>[8x]HHHHHHLEVLFQGPMKYTKLE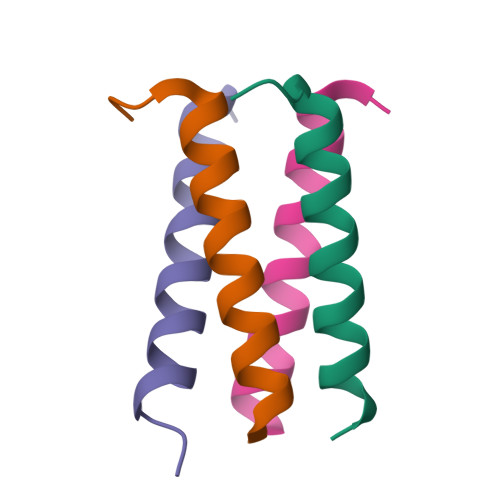KDALDLLSDNEEEDAESSILTFEERDTSSLSIEARLESIEEKLSMILGLLRTLNIATAGPTAARDGIRDAMIGVREELIADIIKEAKGKAAEMMEEE> MADKELKFLVVDDFSTMRRIVRNLLKELGFNNVEEAEDGVDALNKLQAGGYGFVISDWNMPNMDGLELLKTIRADGAMSA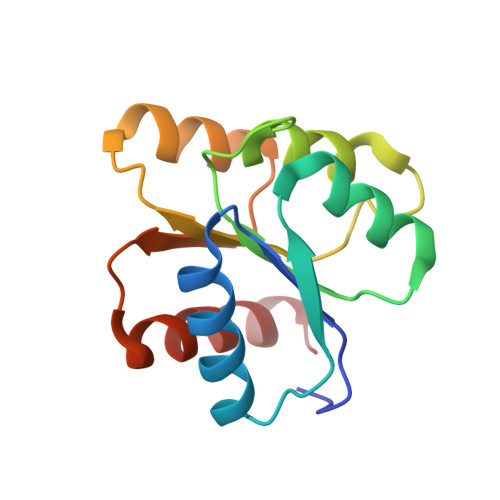LPVLMVTAEAKKENIIAAAQAGASGYVVKPFTAATLEEKLNKIFEKLGM>GSHMEILWNEAKAFIAECYQELGKEEEVKDRLDSIKSEIDLTGSYVHTKEELEHGAKMAWRNSNRCIGRLFWNSLNVIDRRDVRTKEDVRDALFHHIETATNNGKIRPSITIFPPEEKGEKQVEIWNHQLIRYAGYEAAGERIGDPASCSLTAACEQLGWRGERTDFDLLPLIFRMKGDEQPVWYELPRSLVIEVPITHPDIEAFSDLELKWYGVPIISDMKL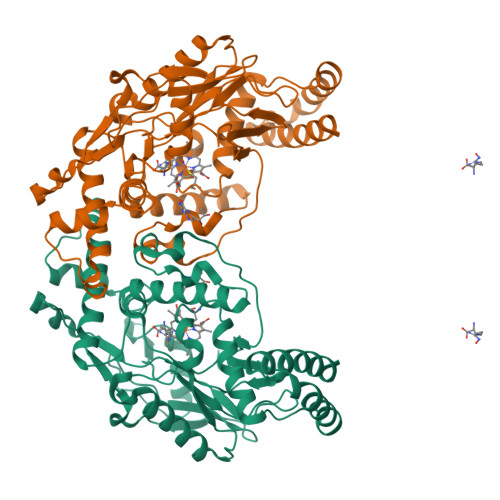EVGGIHYNAAPFNGWYMGTEIGARNLADEKRYDKLKKVASVIGISTNYNTDLWKDQALVELNKAVLYSYKKQGVSIVDHHTAASQFKRFEEQEEEAGRKLTGDWTWLIPPISPAATHIFHRSYDNSIVKPNYFYQDKPYE[2x]>[2x]SNAMGQVRGAAGVTDGNEVAKAQQATPGGAAPTIFSRILDKSLPADILYEDQQCLVFRDVAPQAPVHFLVIPKKPIPRISQA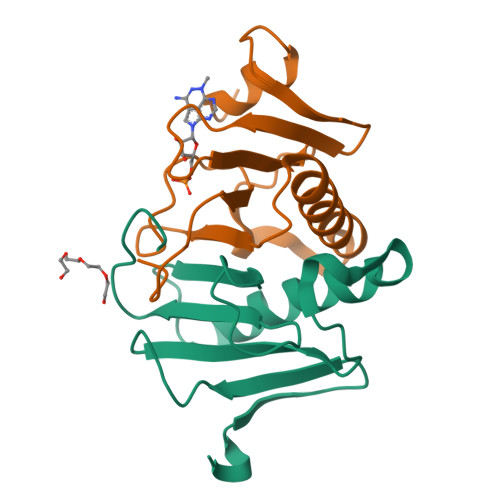EEEDQQLLGHLLLVAKQTAKAEGLGDGYRLVINDGKLGAQSVYHLHIHVLGGRQLQWPPG> SKPFVCANEKDHLPPLDPQADAWYREAAALAKPDTLRPWGRIVEIYSKAVERGHWKAMHNLANLYRTGWPGGVEKDPQKALDLYQKMIDLDVPQGFYDMGAMIGNRAGVKNPATDGLTFLDKAASLGNPPALTELGKLYIYVAKEKELGLAYASCASSQGYAPASYELGSYYELVENNYPKALSYYQVSVSQGGRSAAFFLSRVFGKRTPPSSAMWYTPDEKLEKFYYSLYLQIDADPDLRFPN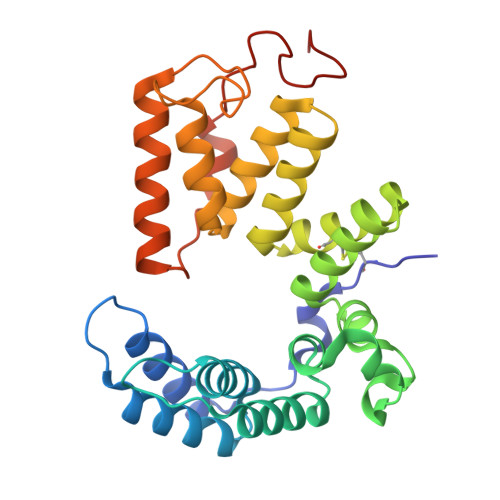LVKYNPLPPHPVQGYDAARPDWKPGQ5-cyclopropyl-2-(5-pyrazin-2-yl-1,2,4-oxadiazol-3-yl)benzo[b][1,4]benzothiazepin-6-one 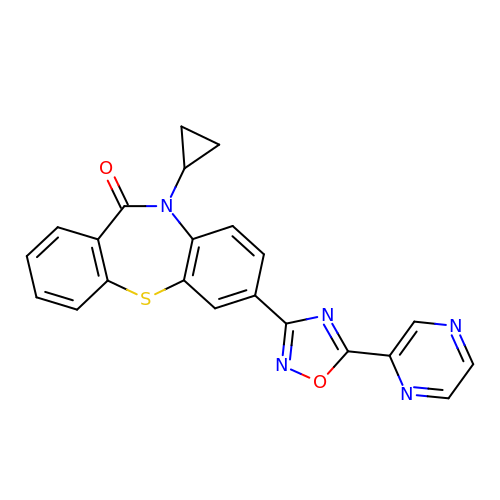| C22 H15 N5 O2 S | ASTXHKRSUWDWQE-UHFFFAOYSA-N>[4x]MASENNGSRSDSESITAPKADSTVVEPRKIALITGITGQDGSYLTEFLLGKGYEVHGLIRRSSNFNTQRIN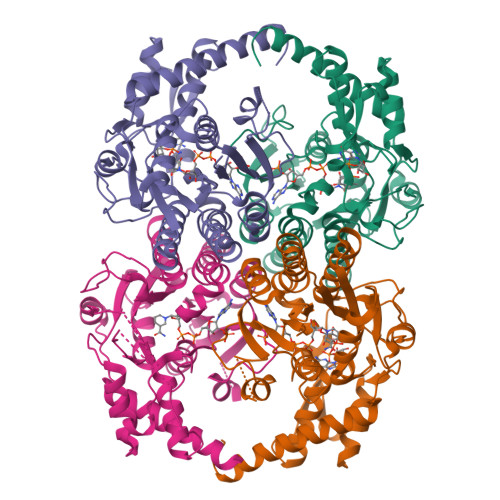HIYIDPHNVNKALMKLHYADLTDASSLRRWIDVIKPDEVYNLAAQSHVAVSFEIPDYTADVVATGALRLLEAVRSHTIDSGRTVKYYQAGSSEMFGSTPPPQSETTPFHPRSPYAASKCAAHWYTVNYREAYGLFACNGILFNHESPRRGENFVTRKITRALGRIKVGLQTKLFLGNLQASRDWGFAGDYVEAMWLMLQQEKPDDYVVATEEGHTVEEFLDVSFGYLGLNWKDYVEIDQRYFRPAEVDNLQGDASKAKEVLGWKPQVGFEKLVKMMVDEDLELAKREKVLVDAGYMDAKQQPLEHHHHHH> GAMDPEFLDPQLPPSSNFDLSAWYLSVPTDNNGDGKADSIKENDLNAGYADGTYFYTAADGGMVFRCPIDGYKTSTNTSYTRTELREMLRRGDTSIATQGVNGNNWVFGSAPASAREAAGGVDGVLRATLAVNHVTTTGDSGQVGRVIVGQIHANNDEPLRLYYRKLPGHSKGSVYIAHEPNGGSDSWYDMIGSRSSSASDPSDGIALDEVWSYEVKVVGNTLTVTIFRAGKDDVVQVVDMGNSGYDVADQYQYFKAGVYNQNNTGNASDYVQVTFYALEQSHD;> 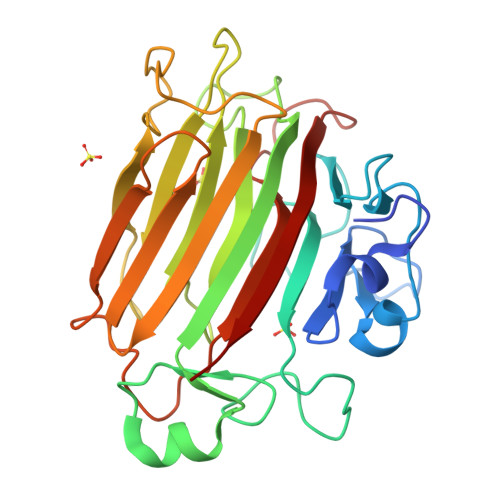GAMDPEFLDPNLPPSSNFDLSAWYLSVPTDNNGDGKADSIKENDLNAGYADGTYFYTAADGGMVFRCPIDGYKTSTNTSYTRTELREMLRRGDTSIATQGVNGNNWVFGSAPASAREAAGGVDGVLRATLAVNHVTTTGDSGQVGRVIVGQIHANNDEPLRLYYRKLPGHSKGSVYIAHEPNGGSDSWYDMIGSRSSSASDPSDGIALDEVWSYEVKVVGNTLTVTIFRAGKDDVVQVVDMGNSGYDVADQYQYFKAGVYNQNNTGNASDYVQVTFYALEQSHD> APRKQLATKAARKSA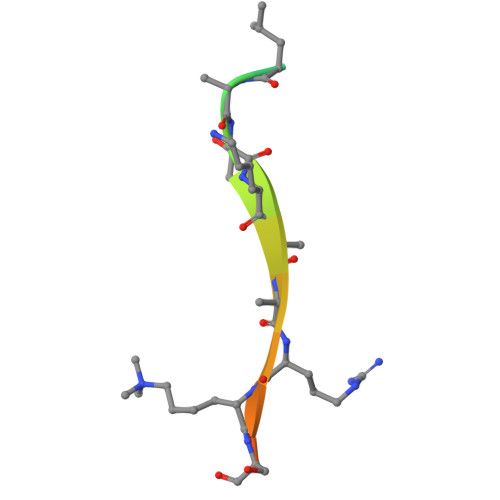PST> LPTSNPAQELEARQLGRTTRDDLINGNSASCRDVIFIYARGSTETGNLGTLGPSIASNLESAFGKDGVWIQGVGGAYRA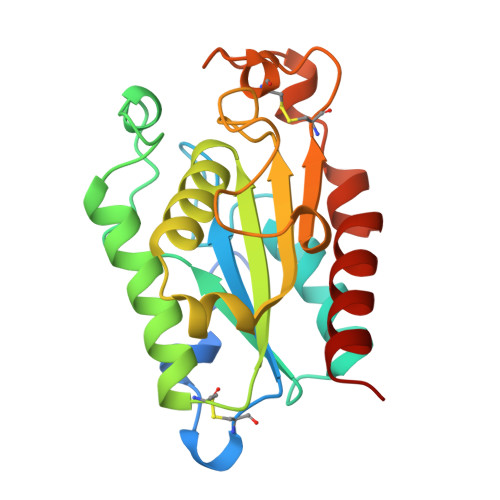TLGDDALPRGTSSAAIREMLGLFQQANTKCPDATLIAGGYSQGAALAAASIEDLDSAIRDKIAGTVLFGYTKNLQNRGRIPNYPADRTKVFCNTGDLVCTGSLIVAAPHLAYGPDARGPAPEFLIEKVRAVRGSA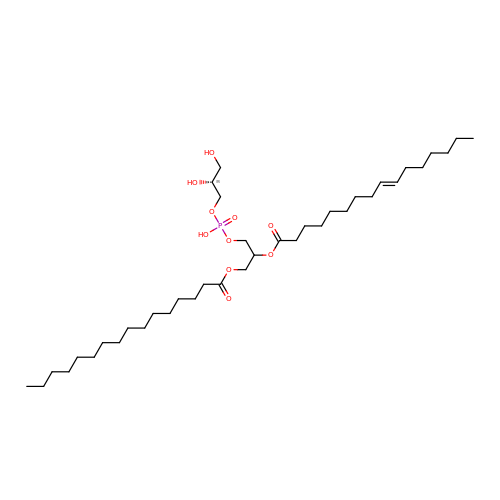[(2~{S})-3-[[(2~{R})-2,3-bis(oxidanyl)propoxy]-oxidanyl-phosphoryl]oxy-2-hexadec-9-enoyloxy-propyl] hexadecanoate | C38 H73 O10 P | NOFOTAHTYLXZNV-RERZGLEZSA-N> SKWRSQLDRFVKENQQDLAALFWGL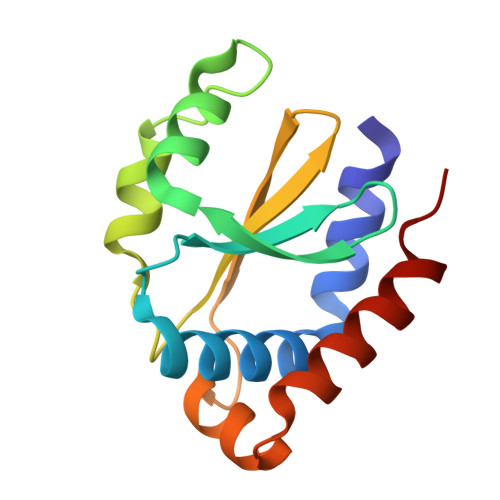WLENGDSQGTIGIDLQPTPHFVYCPKDAVEKLNNNVENRLQELLGIIEHNQPEIEVLMIGIGKGEIKLIQFAPEPPPPVCFEQVGKDIDGLLELLEQRMSGEIVV>MALEPIDYTTHSREIDAEYLKIVRGSDPDTTWLIISPN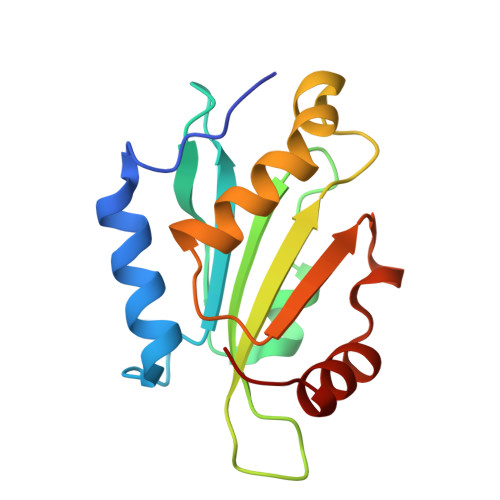AKKEYEPESTGSSFHDFLQLFDETKVQYGLARVSPPGSDVEKIIIIGWCPDSAPLKTRASFAANFAAVANNLFKGYHVQVTARDEDDLDENELLMKISNAAGA[9x]(3S)-3-cyclopentyl-3-[4-(2-{[4-(piperidin-4-yl)phenyl]amino}-7H-pyrrolo[2,3-d]pyrimidin-4-yl)-1H-pyrazol-1-yl]propanenitrile 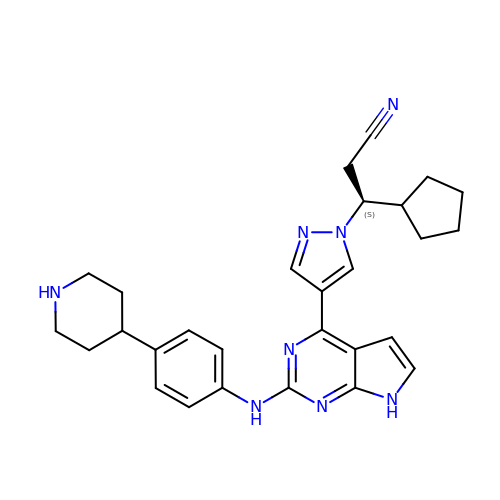| C28 H32 N8 | RGIJZWRVCBSGJV-VWLOTQADSA-N>[2x]GPLGSPPSKEILTLKQ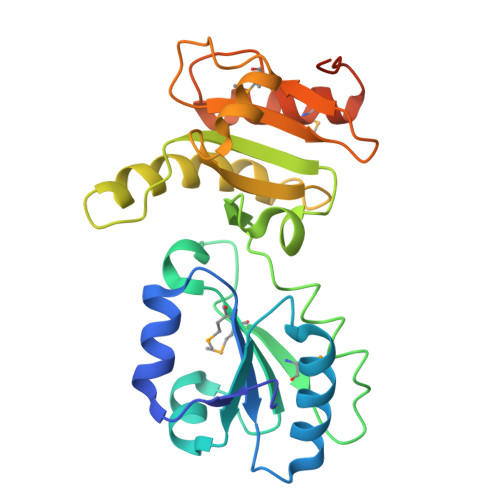VQEFLKDGDDVVILGVFQGVGDPGYLQYQDAANTLREDYKFHHTFSTEIAKFLKVSLGKLVLMQPEKFQSKYEPRMHVMDVQGSTEASAIKDYVVKHALPLVGHRKTSNDAKRYSKRPLVVVYYSVDFSFDYRTATQFWRNKVLEVAKDFPEYTFAIADEEDYATEVKDLGLSESGGDVNAAILDESGKKFAMEPEEFDSDALREFVMAFKKGKLKPVIKSQPVPKNNKGAAAS To understand the molecular basis underlying the superbinding characteristics of the Legionella SH2 domains, we determined the structures of L. longbeachae LeSH and the L. pneumophila RavO SH2 domain in complex with tyrosine-phosphorylated peptides by X-ray crystallography. Compared to the Src SH2 domain, LeSH is missing two β-strands (βA and βF) but contains a 45-residue insert between the strand βE and the helix αB. This extra sequence in LeSH contains a structural motif called the pancreatic polypeptide (PP)-fold, comprising an amphipathic α-helix (named herein as αEF) packed against a polyproline segment via favorable hydrophobic contacts. Indeed, the SH2 and PP folds together form a clamp-like structure that grasp the pTyr residue.

We obtained crystal structures of LeSH in complex with three different pTyr ligands, including the phosphotyrosine itself, a 13-mer peptide derived from the pTyr381 site of DnaJ-A1, and another 13-mer peptide corresponding to the pTyr387 site in IL2Rβ. Apart from the pTyr residue, which assumed the same conformation in all three complexes, we were not able to detect the electron density for residues preceding the pTyr in the DnaJ-A1 peptide or any residues flanking the pTyr in the IL2Rβ peptide despite the high resolution (1.6–1.7 Å) of the complex structures obtained. This suggests that, in contrary to their important role in binding to a mammalian SH2 domain, residues C-terminal to the pTyr may not make a significant contribution in binding to a Legionella SH2 domain. Of note, the positive charge on LeSH extends well beyond the pTyr-binding pocket due to the presence of a Lys-rich face in the αEF helix. The expansive positive electrostatic potential explains the general (i.e., position-independent) preference for acidic residues by LeSH beyond the pTyr. However, the R46K mutant of LeSH bound the DnaJ-A1 and IL2βR peptides that contain multiple Asp/Glu residues markedly better than to the remaining peptides that contain fewer acidic residues. This indicates that charge–charge interaction plays a pivotal role in the LeSH-peptide ligand interaction.

> GAMEAMQKNELNSKIPIIFGLINSYQIHNLLEQHNAKTKESKAVFLIRDSSTYPGLLTISYYCQEQDIVKHIRFGLTDKGWKTAPKPPHEPLKSDSPEIKEKYTLDKIKFERKMKQFINTAKKLFEQHIRAESFKTLIMELKIHEFNLEGLIKPTRSQASQEKHFTDYV;> YFTYDPYSEEDPD>GSSPEKPTPNGGIPHDNLV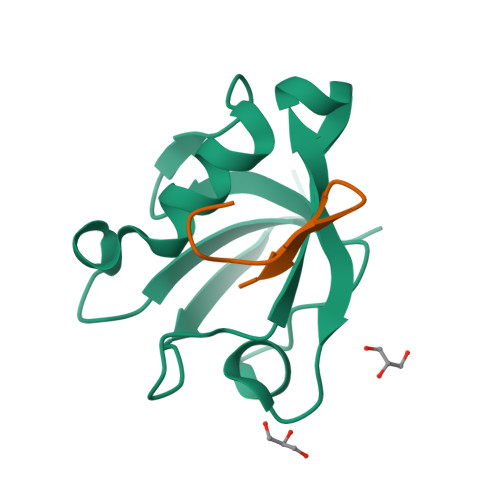LIRMKPDENGRFGFNVKGGYDQKMPVIVSRVAPGTPADLCVPRLNEGDQVVLINGRDIAEHTHDQVVLFIKASCERHSGELMLLVRPN[2x];>[2x]SWESHKSGGETRL> MTFTVDITPKTPTGVIDETKQFTATPSGQTGGGTITYAWSVDNVPQDGAEATFSYVLKGPAGQKTIKVVATNTLSEGGPETAEATTTITVKNKTQTTTLAVTPASPAAGVIGTPVQFTAALASQPDGASATYQWYVDDSQVGGETNSTFSYTPTTSGVKRIKCVAQVTATDYDALSVTSNEVSLTVNKKTMNPQVTLTPPSINVQQDASATFTANVTGAPEEAQITYSWKKDSSPVEGSTNVYT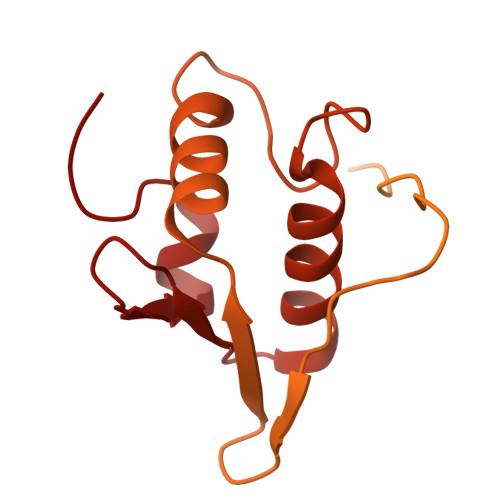VDTSSVGSQTIEVTATVTAADYNPVTVTKTGNVTVTAKVAPEPEGELPYVHPLPHRSSAYIWCGWWVMDEIQKMTEEGKDWKTDDPDSKYYLHRYTLQKMMKDYPEVDVQESRNGYIIHKTALETGIIYTYP> ASSRLVQSTLDQFIPYKGWKLYFSEAYADKSPFVQKTQAFEKFFMQRIELYDKDEIERKGSILVDYKELIEDRELTKSIPNISTELRDMPQKILQC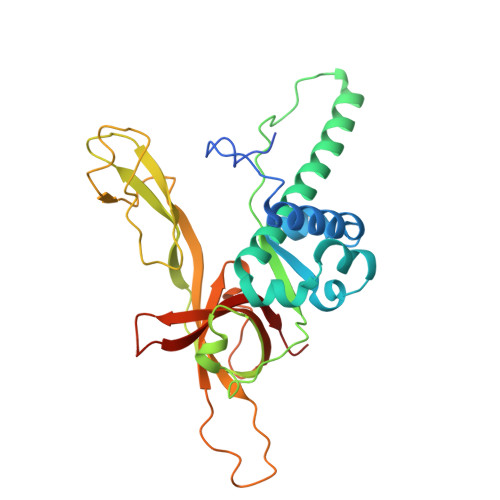MGLAIHQVLTKDLERHAAELQVQEGLPLDGEPIINVPLIHARLYNYEPLTQLKNVRANCYGKYIALRGTVVRVSNIKPLCTKLAFVCGTCGDVQSVPLPDGKYTLPTKCLVPECRGRSFTPDRSSPLTATVDWQSVKVQELMSDDQREAGRIPRTIECELVQDLVDSCVPGDVVTITGVVKVSSTEEGASKNKNDKCVFLLYIEANSVSNSK>MTTSASSHLNKGIKQVYMSLPQGEKVQAMYIWIDGTGEGLRCKTRTLDSEPKCVEELPEWNFDGSSTLQSEGSNSDMYLVPAAMFRDPFRKDPNKLVLCEVFKYNRRPAETNLRHTCKRIMDMVSNQHPWFGMEQEYTLMGTDGHPFGWPSNGFPGPQGPYYCGVGADRAYGRDIVEAHYRACLYAGVKIAGTNAEVMPAQWEFQIGPCEGISMGDHLWVARFILHRVCEDFGVIATFDPKPIPGNWNGAGCHTNFSTKAMREENGLKYIEEAIEKLSKRHQYHIRAYDPKGGLDNARRLTGFHETSNINDFSAGVANRSASIRIPRTVGQEKKGYFEDRRPSANCDPFSVTEALIRTCLLNETGDEPFQYKN[20x]

Glutamine synthetase (GS) is an ancient enzyme that catalyzes the ATP-dependent condensation of glutamate and ammonia to glutamine (Eisenberg et al. 2000; de Carvalho Fernandes, Turchetto-Zolet, and Pereira Passaglia 2022; Tecson et al. 2025). Here, we demonstrate that human glutamine synthetase (GS) can reversibly polymerize into filaments aided by a composite binding site formed at the filament interface by the product, glutamine. The glutamate/ammonia binding site is gated by a flexible loop that bears two key catalytic residues: R299, which interacts with glutamate substrate carboxyl group, and E305, which is predicted to deprotonate ammonium ions to ammonia, enabling the required nucleophilic attack of the y-glutamyl phosphate intermediate. We propose that GS filament formation constitutes a negative-feedback mechanism, directly linking product concentration to the structural and functional remodeling of the enzyme.

We performed an additional cryoEM experiment with increased GS concentration (1.5 mg/mL), to bias our particle populations towards filamentous assemblies, and vitrified at 57s, a reaction time that should yield a high concentration of product due to the higher enzyme concentration than previous experiments. The resulting 3D reconstruction of the 2-decameric species had an FSC 0.143 of 2.2Å. Inspection of the ‘filament assembly’ interface between the two decamers revealed a discrete density that was absent from the apo-filament reconstruction. The density is too small for a nucleotide (ATP or ADP) and too large for inorganic phosphate. Given the association with product formation, we modeled glutamine into this density in a conformation consistent with forming hydrogen bonds that link the filament interface residues and the bound product. The two-fold symmetry at this interface and the averaging inherent in our data processing results in density that likely reflects contributions from glutamine in two orientations. Taken together, these data support a model wherein glutamine synthetase filamentation generates a composite binding site for glutamine at the filament interface, which is located over 10Å from the active site. By contrast, the filament map collected during turnover displayed almost no density in the region, which is indicative of a greater degree of disorder. However, the turnover-filament model displays distended loop conformations diverged from the active-closed state that we turn collectively as the ‘open ensemble’ of loop conformations. The E305-loop (residues 299 – 311) sampled a more diverse ensemble (with root mean square fluctuation values of greater than 10Å) in the turnover filament state, with the turnover decamer and apo-filament displaying reduced variability.> GSKNTSGDLSQKQALQLALSAREHFWNTMSGHNPKVKKAVCPSGTFEYQNLQYVYMCSDLGTKAKAVNYLTPIFTKTAIEKGFKDYHFTVSKGKL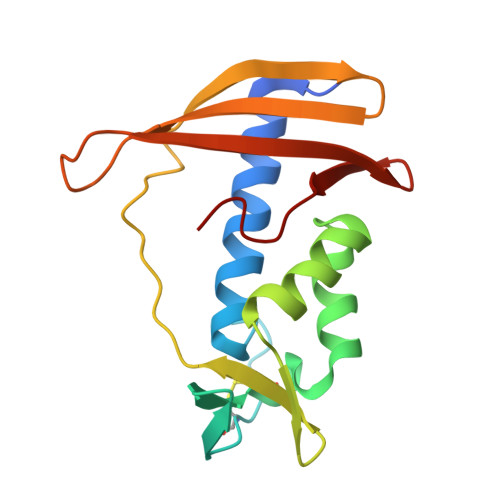AVPIGDGDNLLNWKKSTAKLISKKGSTITYEFTVPTLDGSPSAKRKVTFVKENKKWKVNQFDAVI>[2x]MDHLPIFCQLRDRDCLIVGGGDVAERKARLLLEAGARLTVNALTFIPQFTVWANEGMLTLVEGPFDETLLDSCWLAIAATDDDTVNQRVSDAAESRRIFCNVVDAPKAASFIMPSIIDRSPLMVAVSAGGTSPVLARLLREKLESLLPQHLGQVARYAGQLRARVKKQFATMGERRRFWEKFFVNDRLAQSLANADEKAVNATTERLFSEPLDHRGEVVLVGAGPGDAGLLTLKGLQQIQQADIV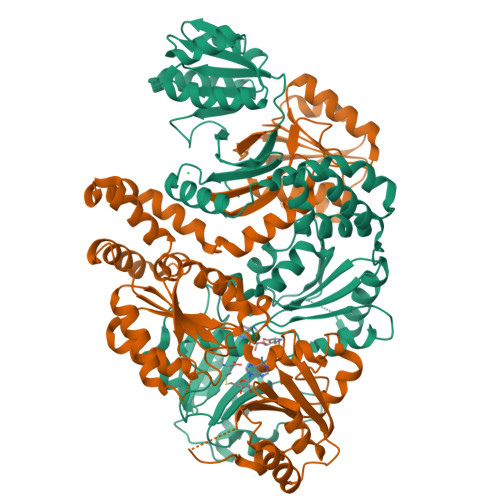VYDRLVSDDIMNLVARDADRVFVGKRAGYHCVPQEEINQILLREAQKGKRVVRLKGGDPFIFGRGGEELETLCHAGIPFSVVPGITAASGCSAYSGIPLTHRDYAQSVRLVTGHLKTGGELDWENLAAEKQTLVFYMGLNQAATIQEKLIAFGMQADMPVALVENGTSVKQRVVHGVLTQLGELAQQVESPALIIVGRVVALRDKLNWFSNH>MKVWNARNDHLTINQWATRIDEILEAPDGGEVIYNVDENDPREYDAIFIGGGAAGRFGSAYLRAMGGRQLIVDRWPFLGGSCPHNACVPHHLFSDCAAELMLARTFSGQYWFPDMTEKVVGIKEVVDLFRAGRNGPHGIMNFQSKEQLNLEYILNC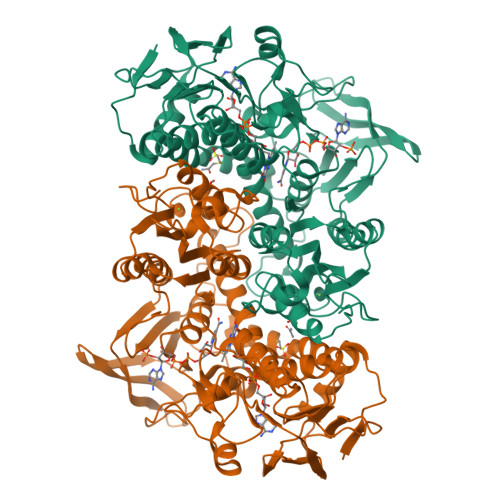PAKVIDNHTVEAAGKVFKAKNLILAVGAGPGTLDVPGVNAKGVFDHATLVEELDYEPGSTVVVVGGSKTAVEYGCFFNATGRRTVMLVRTEPLKLIKDNETRAYVLDRMKEQGMEIISGSNVTRIEEDANGRVQAVVAMTPNGEMRIETDFVFLGLGEQPRSAELAKILGLDLGPKGEVLVNEYLQTSVPNVYAVGDLIGGPMEMFKARKSGCYAARNVMGEKISYTPKNYPDFLHTHYEVSFLGMGEEEARAAGHEIVTIKMPPDTENGLNVALPASDRTMLYAFGKGTAHMSGFQKIVIDAKTRKVLGAHHVGYGAKDAFQYLNVLIKQGLTVDELGDMDELFLNPTHFIQLSRLRAGSKNLVSL[2x]>[4x]GIDPFTAKRTHRVINHPYYFPFNGRQAEDYLRSKERGEFVIRQSSRGDDHLVITWKLDKDLFQHIDIQELEKENPLALGKVLIVDNQKYN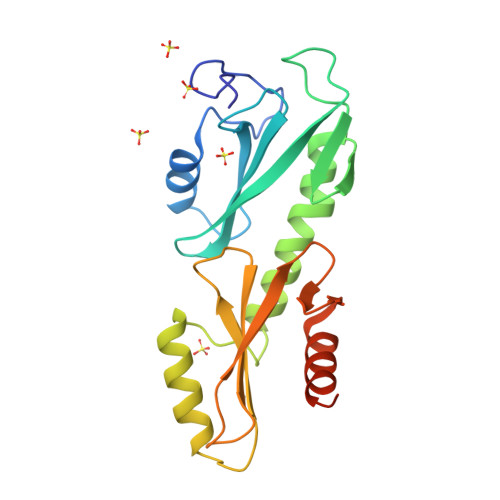DLDQIIVEYLQNKVRLLNEMTSSEKFKSGTKKDVVKFIEDYSRVNPNKSVYYFSLNHDNPGWFYLMFKINANSKLYTWNVKLTNTGYFLVNYNYPSVIQLCNGFKTLLKSNSSKNRMNNYR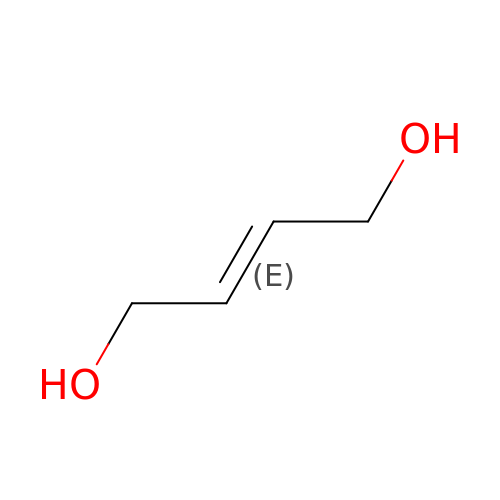(2E)-but-2-ene-1,4-diol | C4 H8 O2 | ORTVZLZNOYNASJ-OWOJBTEDSA-N>[6x]GSSPN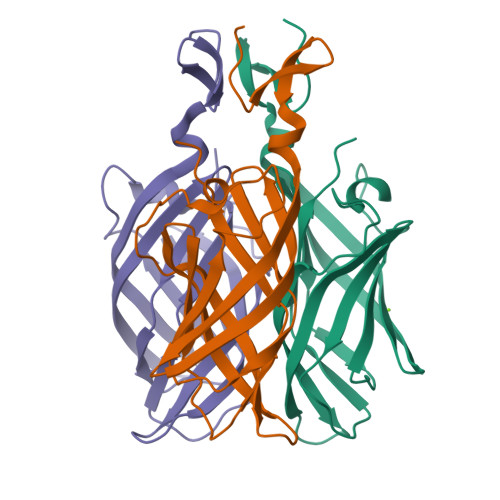LRYPIADVSGGIGMSPNYRFRQSMWIGIVSYSGSGLNWRVQVNSDIFIVNDYIHICLPAFDGFSIADGGDLSLNFVTGLLPPLLTGDTEPAFHNDVVTYGAQTVAIGLSSGGTPQYMSKNLWVEQWQDGVLRLRVEGGGSITHSNSKWPAMTVSYPRSFT>[2x]MSARILVVDDIEANVRLLEAKLTAEYYEVSTAMDGPTALAMAARDLPDIILLDVMMPGMDGFTVCRKLKDDPTTRHIPVVLITALDGRGDRIQGLESGASDFLTKPIDDVMLFARVRSLTRFKLVIDELRQREASGRRMGVIAGAAARLDGLGGRVLIVDDNERQAQRVAAELGVEHRPVIESDPEKAKISAGGPVDLVIVNAAAKNFDGLRFTAALRSEERTRQLPVLAMVDPDD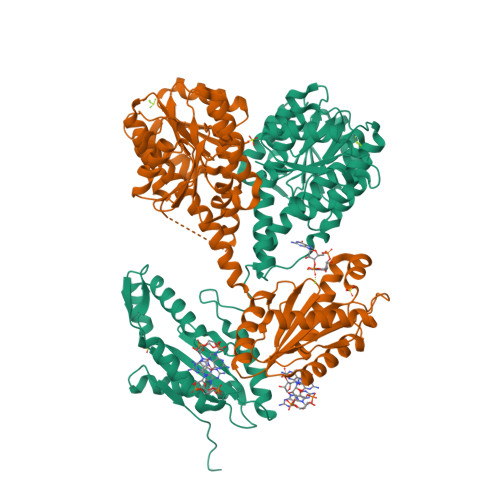RGRMVKALEIGVNDILSRPIDPQELSARVKTQIQRKRYTDYLRNNLDHSLELAVTDQLTGLHNRRYMTGQLDSLVKRATLGGDPVSALLIDIDFFKKINDTFGHDIGDEVLREFALRLASNVRAIDLPCRYGGEEFVVIMPDTALADALRIAERIRMHVSGSPFTVAHGREMLNVTISIGVSATAGEGDTPEALLKRADEGVYQAKASGRNAVVGKAAHHHHH>ETGESLAKETAFVEVVLFESSPNGDYKTHTTELQGRFSRAGATISAEGEIVQMHPLGLCNNNDEEDLYEYGWVGVVKLEQPEMDPKPCLTVLGKAKRAVQRGATAVIFDVSDNPDAVEQLNQGLEDPLKRPVVYMKGMDAIKLMNIVNKQKGARARIQHRPPRQPTEYFDGTHHHHHHHHHH[2x];>[2x]ETGGTNPICKGCLSCSKDNGCLRCQPKLFFYLRREGMRQYGECLQSCPPGYYGVRGPDMNRCSRCRIENCDSCFSRDFCIKCKSGFYSHKGQCFEECPEGFAPLDDTMVCVDGTKHHHHHH

Rspo (R-spondin, also roof plate-specific spondin) proteins are evolutionarily conserved from fish to humans and have well-documented roles in a broad range of developmental and physiological processes resulting from enhancement of canonical and non-canonical Wnt signalling. ZNRF3/RNF43 specifically targets these Wnt receptors for ubiquitination and turnover, hence reducing Wnt signalling responses. Direct extracellular interaction with Rspo proteins inhibits ZNRF3/RNF43 activity. Here we report a molecular level analysis of the ZNRF3/RNF43 ectodomain structure and its interactions with Rspo proteins.

By using a combination of heavy atom and molecular-replacement-based phasing strategies, we determined multiple crystal structures for Xenopus (x) Rspo2Fu1–Fu2 (highest resolution 2.2 Å), xZNRF3ecto, zebrafish (z) ZNRF3ecto and mouse (m) ZNRF3ecto, (highest resolutions 2.4, 1.6 and 2.0 Å, respectively), plus complexes comprising xZNRF3ecto–xRspo2Fu1–Fu2, mZNRF3ecto–mRspo2Fu1–Fu2, mZNRF3ecto–xRspo2Fu1–Fu2 and xRNF4F3ecto–xRspo2Fu1–Fu2 (at 2.1, 2.8, 2.4 and 2.7 Å, respectively). The crystal structures of the ZNRF3ecto–Rspo2Fu1–Fu2 and RNF43ecto–Rspo2Fu1–Fu2 complexes revealed a 1:1 interaction between Fu1 of the Rspo2Fu1–Fu2 and a single ZNRF3ecto or RNF43ecto chain. Neither the Rspo2Fu1–Fu2 nor the ZNRF3ecto dimer show major conformational changes on complex formation. The first, extensive, area of interaction involves hydrophobic interactions interspersed with hydrophilic (complementarily charged) patches contributed by the first two β-hairpins of the Rspo Fu1 and the region immediately carboxy-terminal to the β3 strand of ZNRF3ecto. The Met-finger at the tip of the second β-hairpin of Fu1 nestles into a pocket formed between the β3 strand and the αC–β7 loop of the ZNRF3ecto, which is lined with hydrophobic residues (I95, I191, V192, A198). The αC–β7 loop is a flexible region in the unliganded ZNRF3ecto crystal structures and moulds to interface the RspoFu1–Fu2 M68 in the complex. The acidic region of the β3–β4 loop (immediately adjacent to C104 of the disulphide bridge) becomes more ordered in the ligand-bound ZNRF3ecto structures, probably as a result of electrostatic interactions with a positively charged patch on Rspo Fu1. For all ZNRF3ecto–Rspo2Fu1–Fu2 complex structures we determined (from five different combinations of species and crystal forms), the dimer found in most of the unliganded ZNRF3ecto crystal structures reoccurs. The overall assembly thus comprises a 2:2 complex of ZNRF3ecto–Rspo2Fu1–Fu2. The 2:2 complex resembles a crab with the ZNRF3ecto dimer forming the body from which the two Rspo2Fu1–Fu2 ligands diverge, without interacting with each other, as the pincers.> MRDAVTTLIKNYDLTGRYLDRNAMDELKAYFESGSARIAAAAMINANSATIVKRA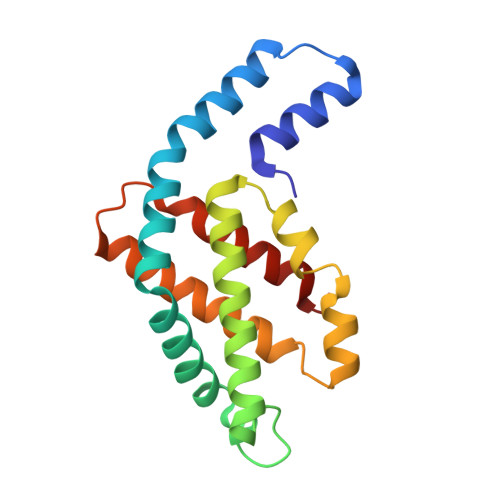AAQLFEEIPELIRPSGNAYTTRRFSACLRDMDYYLRYASYALIAADNNVLDERVLQGLRETYNSLGVPIGPTVRGIQIMKEMIEAMAEDSSLNSTDFIASPFDHMTRELSELSV> GAMVIEKEDVETNASNGQRVDLSSELDKLKKLENATVHMEFK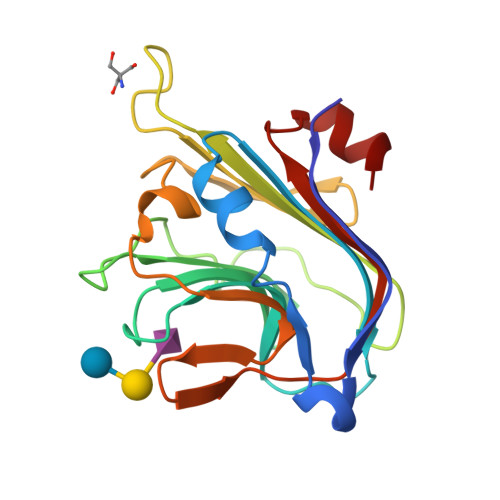PDAKAPAFYNLFSVSSATKKDEYFTMAVYNNTATLEGRGSDGKQFYNNYNDAPLKVKPGQWNSVTFTVEKPTAELPKGRVRLYVNGVLSRTSLRSGNFIKDMPDVTHVQIGATKRANNTVWGSNLQIRNLTVYNRALTPEEVQKRS> SVLQVLHIPDERLRKVAKPVEEVNAEIQRIVDDMFETMYAEEGIGLAATQVDIHQRIIVIDVSENRDERLVLINPELLEKSGETGIEEGCLSIPEQRALVPRAEKVKIRALDRDGKPFELEADGLLAICIQHEMDHLVGKLFM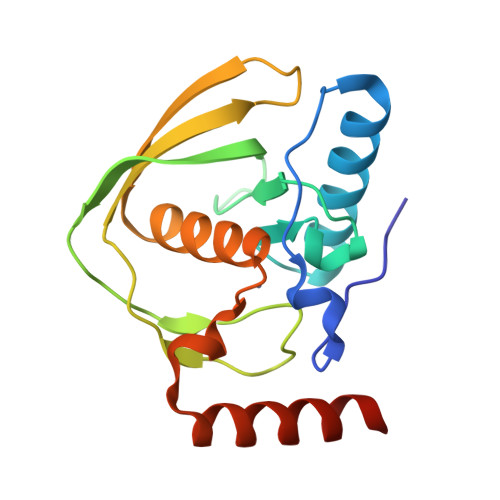DYLSPLKQQRIRQKVEKLDRLKARA>[14x]KMLEGQNAHFRYKNR;>[14x]GSHMAKYTREDIEKLVKEENVKYIRLQFTDILGTIKNVEIPVSQLGKALDNKVMFDGSSIEGFVRIEESDMYLYPDLNTFVIFPWTAEKGKVARFICDIYNPDGTPFEGDPRNNLKRILKEMEDLGFSDFNLGPEPEFFLFKLDE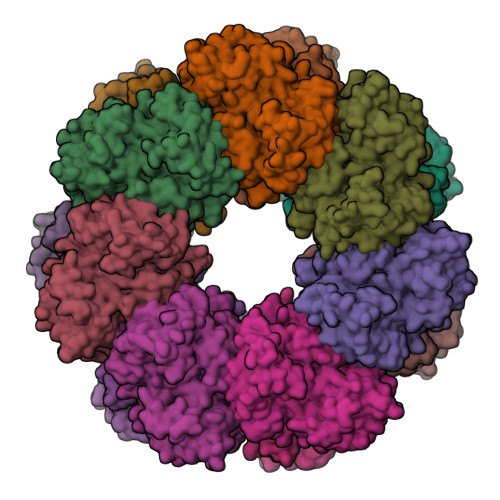KGEPTLELNDKGGYFDLAPTDLGENCRRDIVLELEEMGFEIEASHHEVAPGQHEIDFKYAGAVRSCDDIQTFKLVVKTIARKHGLHATFMPKPLFGVNGSGMHCNLSLFKNGVNAFFDENADLQLSETAKHFIAGIVKHATSFTAVTNPTVNSYKRLVPGYEAPCYVAWSAQNRSPLIRIPASRGISTRVEVRSVDPAANPYLALSVLLAAGLDGIKNKLEAPAPIDRNIYVMSKEERMENGIVDLPATLAEALEEFKSNEVMVKALGEHLFEHFIEAKEIEWDMFRTQVHPWEREQYMSQY>[2x]MEDSLYSLLVAELAGQRNRFDIALSNYVVQAQKTRDPGVSERAFRIAEYLGADQEALDTSLLWARSAPDNLDAQRAAAIQLARAGRYEESMVYMEKVLNGQGDTHFDFLALSAAETDPDTRAGLLQSFDHLLKKYPNNGQLLFGKALLLQQDGRPDEALTLLEDNSASRHEVAPLLLRSRLLQSMKRSDEALPLLKAGIKEHPDDKRVRLAYARLLVEQNRLDDAKAEFAGLVQQFPDDDDLRFSLALVCLEAQAWDEARIYLEELVERDSHVDAAHFNLGRLAEEQKDTARALDEYAQVGPGNDFLPAQLRQTDVLLKAGRVDEAAQRLDKARSEQPDYAIQLYLIEAEALSNNDQQEKAWQAIQEGLKQYPEDLNLLYTRSMLAEKRNDLAQMEKDLRFVIAREPDNAMALNALGYTLADRTTRYGEARELILKAHKLNPDDPAILDSMGWINYRQGKLADAERYLRQALQRYPDHEVAAHLGEVLWAQGRQGDARAIWREYLDKQPDSDVLRRTIKRLTGAETPKLAAALEHHHHHH

Pseudomonas aeruginosa CtpA is a carboxyl-terminal processing protease that partners with the outer membrane lipoprotein LbcA to degrade at least five cell wall-associated proteins, four of which are cell wall hydrolases. Instead, it requires the adaptor protein LbcA, the lipoprotein-binding partner of CtpA, for activity in vivo and in vitro. Therefore, it appears that LbcA interacts with CtpA to assemble an active proteolytic complex, which controls the activity of these enzymes by degrading them. We show that CtpA alone assembles as an inactive trimer of dimers and that LbcA is a right-handed spiral that might wrap around a substrate protein.

We were able to crystallize LbcA with its N-terminal 48 residues removed (ΔN48). The crystal structure was solved to 3.5-Å resolution by the SAD method with selenomethionine-derivatized LbcA(ΔN48) crystals. This structure contains only α-helices and connecting loops, with a total of 29 α-helices. We resolved all 11 predicted tetratricopeptide repeats, comprising 22 α-helices from helix 7 (H7) to H28. The 11 TPRs form a notched ring, with an outer diameter of about 6 nm and an inner diameter of about 3 nm. It is a right-handed spiral structure, because the first TPR is slightly above the ring, and the last TPR is below the ring. The first four α-helices at the N terminus form an elongated extension that partially caps the TPR ring. However, four LbcA(ΔN48) molecules formed an interlocked tetramer as a dimer of dimers in the crystal. The chamber of the TPR spiral of the first LbcA is occupied by the H1-H4 of a second LbcA molecule on the top and by the H2-H3 of a third LbcA molecule on the side. We suggest that this bundle may mimic a substrate and that the LbcA spiral may wrap around a substrate to target it to CtpA for degradation.> MAQIQRVALFPHATFHIALARVFGLGKSTSLAVSEACGISKDLKVKD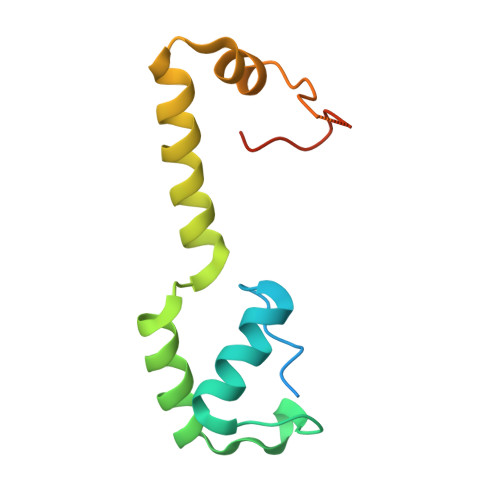VKDSYIQKVTAYIEANFVTGDTLKRQVRENVLEEVAINSRRGVRHTLGLPVSSAQTRSNGVNARKLRPLLLYDTSRR>TGHNTTVFQGVAGQSLQVSCPYDSMKHWGRRKAWCRQLGEKGPCQRVVSTHNLWLLSFLRRWNGSTAITDDTLGGTLTITLRNLQPHDAGLYQCQSLHGSEADTLRKVLVEVLADPLGTKHHHHHH[2x]

TREM2 is an innate immune receptor expressed on dendritic cells (DCs), resident macrophages such as osteoclasts and microglia, infiltrating and inflammatory macrophages, and CSF monocytes (Colonna and Wang, 2016). It is a type one receptor protein consisting of an extracellular V-type Ig domain, a short stalk, a transmembrane domain that associates with the adaptor protein DAP12 for signaling, and a cytoplasmic tail. For example, whole genome and whole exome sequencing has identified point mutations in the gene encoding the protein TREM2 (triggering receptor expressed on myeloid cells 2) that correlate with a significantly increased risk of developing Alzheimer’s disease (AD). We found that NHD-causing mutations impact TREM2 protein folding and stability, whereas AD risk variants decrease binding to the cellular TREM2-ligand (TREM2-L).

We previously reported the crystallization of the WT human TREM2 ectodomain (amino acids 19–134) purified from a mammalian cell expression system. We determined the crystal structure of the TREM2 ectodomain at 3.1 Å resolution and found that the disease-linked mutations exhibit distinct structural patterns, suggesting that they would impact TREM2 function through alternate mechanisms. The TREM2 ectodomain is a V-type Ig domain containing two disulfide bonds, the canonical Ig disulfide between residues C36 and C110 (βB–βF) and an additional linkage between C51 and C60 (βC-βC’). A single N-acetylglucosamine (NAG) glycan that remains after Endo Hf treatment is clearly visible in the electron density at residue N79. The nine β-strands characteristic of proteins within this Ig domain class are present, and two short α-helix passages are observed spanning β-sheets B–C and E–F. The asymmetric unit (ASU) contains two monomers of hTREM2 in a parallel arrangement, but the limited buried surface area (~400 Å2) and chemical nature of the interface suggest that this dimer would not exist in solution. The side chains of mutations causing NHD (Y38, T66 and V126) are all buried within the core of the Ig fold, whereas the side chains of verified AD risk variants (R47H and R62H) and possible AD risk variants (N68K, D87N and T96K) all lie on the protein surface. R47, the residue with the strongest link to AD as the R47H variant, is at the end of the loop preceding β-sheet C. It is well-ordered in the structure with the side chain lying parallel along the surface of the protein, and the side-chain amines engage the carbonyl oxygen of T66. Indeed, anionic bacterial carbohydrates, phospholipids, myelin lipids, and even purified DNA all activate TREM2 reporter cell lines. This is not surprising in light of our crystal structure, which reveals an extended basic patch on the surface of TREM2 that would be capable of forming electrostatic interactions with these anionic ligands.(2S)-2-AMINO-2-BENZYL-3-HYDROXYPROPYL 3-({[(1R)-1-(4-FLUOROPHENYL)ETHYL]AMINO}CARBONYL)-5-[METHYL(METHYLSULFONYL)AMINO]BENZOATE | C28 H32 F N3 O6 S | 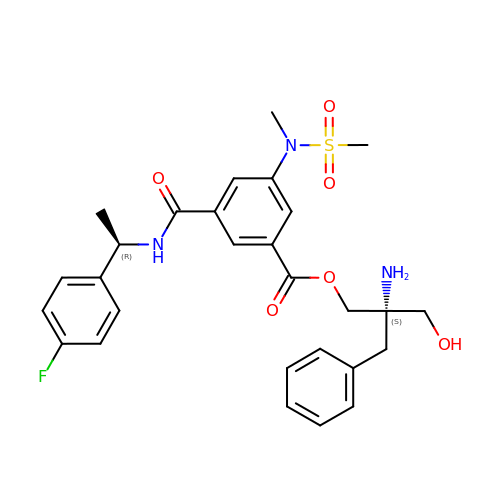JVYHUOIVVLDSHT-GDJIYFAZSA-N>[3x]SAWRKAGISYAAYLNVAAQAIRSSLKTELQTASVLNRSQTDAFYTQYKNGTAASEPTPITK;>[9x]ASTKAQPTEVSSILEERIKGVSDEANLNETGRVLAVGDGIARVFGLNNIQAEELVEFSSGVKGMALNLEPGQVGIVLFGSDRLVKEGELVKRTGNIVDVPVGPGLLGRVVDALGNPIDGKGPIDAAGRSRAQVKAPGILPRRSVHEPVQTGLKAVDALVPIGRGQRELIIGDRQTGKTAVALDTILNQKRWNNGSDESKKLYCVYVAVGQKRSTVAQLVQTLEQHDAMKYSIIVAATASEAAPLQYLAPFTAASIGEWFRDNGKHALIVYDDLSKQAVAYRQLSLLLRRPPGREAYPGDVFYLHSRLLERAAKLSEKEGSGSLTALPVIETQGGDVSAYIPTNVISITDGQIFLEAELFYKGIRPAINVGLSVSRVGSAAQVKALKQVAGSLKLFLAQYREVAAFAQFGSDLDASTKQTLVRGERLTQLLKQNQYSPLATEEQVPLIYAGVNGHLDGIELSRIGEFESSFLSYLKSNHNELLTEIREKGELSKELLASLKSATESFVATF;>ASAAQSTPITGKVTAVIGAIVDVHFEQSELPAILNALEIKTPQGKLVLEVAQHLGENTVRTIAMDGTEGLVRGEKVLDTGGPISVPVGRETLGRIINVIGEPIDERGPIKSKL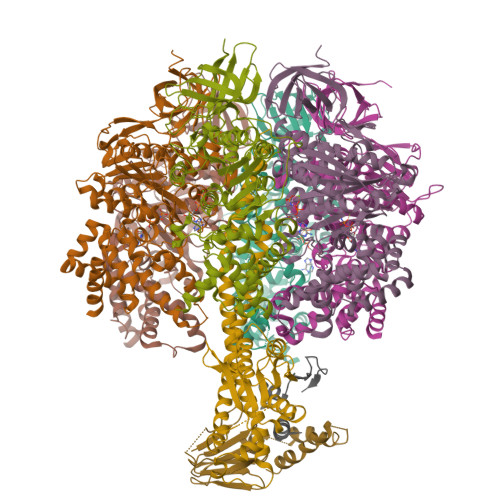RKPIHADPPSFAEQSTSAEILETGIKVVDLLAPYARGGKIGLFGGAGVGKTVFIQELINNIAKAHGGFSVFTGVGERTREGNDLYREMKETGVINLEGESKVALVFGQMNEPPGARARVALTGLTIAEYFRDEEGQDVLLFIDNIFRFTQAGSEVSALLGRIPSAVGYQPTLATDMGLLQERITTTKKGSVTSVQAVYVPADDLTDPAPATTFAHLDATTVLSRGISELGIYPAVDPLDSKSRLLDAAVVGQEHYDVASKVQETLQTYKSLQDIIAILGMDELSEQDKLTVERARKIQRFLSQPFAVAEVFTGIPGKLVRLKDTVASFKAVLEGKYDNIPEHAFYMVGGIEDVVAKAEKLAAEAN[9x];>[3x]ATLKEVEMRLKSIKNIEKITKTMKIVASTRLSKAEKAKISAKKMDEAEQLFYKNAETKNLDVEATETGAPKELIVAITSDKGLCGSIHSQLAKAVRRHLNDQPNADIVTIGDKIKMQLLRTHPNNIKLSINGIGKDAPTFQESALIADKLLSVMKAGTYPKISIFYNDPVSSLSFEPSEKPIFNAKTIEQSPSFGKFEIDTDANVPRDLFEYTLANQMLTAMAQGYAAEISARRNAMDNASKNAGDMINRYSILYNRTRQAVITNELVDIITGASSLG;>AEAAAASSGLKLQFALPHETLYSGSEVTQVNLPAKSGRIGVLANHVPTVEQLLPGVVEVMEGSNSKKFFISGGFATVQPDSQLCVTAIEAFPLESFSQENIKNLLAEAKKNVSSSDAREAAEAAIQVEVLENLQSVLK[3x]> ADLGHQTLGSNDGWGAYSTGTTGGSKASSSNVYTVSNRNQLVSALGKETNTTPKIIYIKGTIDMNVDDNLKPLGLNDYKDPEYDLDKYLKAYDPSTWGKKEPSGTQEEARARSQKNQKARVMVDIPANTTIVGSGTNAKVVGGNFQIKSDNVIIRN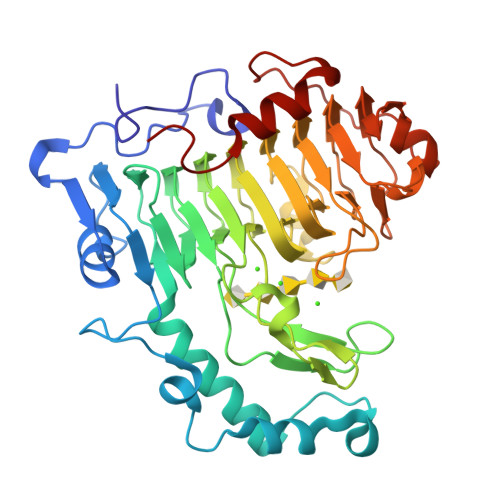IEFQDAYDYFPQWDPTDGSSGNWNSQYDNITINGGTHIWIDHCTFNDGSRPDSTSPKYYGRKYQHHDGQTDASNGANYITMSYNYYHDHDKSSIFGSSDSKTSDDGKLKITLHHNRYKNIVQAAPRVRFGQVHVYNNYYEGSTSSSSYPFSYAWGIGKSSKIYAQNNVIDVPGLSAAKTISVFSGGTALYDSGTLLNGTQINASAANGLSSSVGWTPSLHGSIDASANVKSNVINQAGAGKLN> MDRFQIGDEQLLRFYQLKTINPTHSWAQDSSKLNNEEATSNELGVETSFDILKDFKYGNQISIDKESRAYLNDESLSYIRDPLNGQEMSKELQHLPNDSMRLNYLVNSKQFNVKAFLRDMHKQDSFNDLNNSLDRLDSDIQDQSIHLKQLVGKNFTKYVKIKNKLDQIYKEFDEKTNEKNQCDSPKENQINVESLNKKVDEVIRTTTFKLKPLMDNYQKILNYQATKKFIELNKFYFNLPKSLKRCLTNNDFNEFIIEYSKGLTLRRRFNQSSDASQSLVIKRIWTQIENLLVTYKDLIWNSLINSNFNIDQPQETILSLFSKLLNLENFINNNQRESESGNKNTTSSSNENPILRWMSIKMNGFQNELNELSGHMISKIIHSQRLILQNNTNQDKSQGCVELSYYLKINQLFQIISDTGKDSEGLKSTVEPNKVNTISGTSYLNLNCQPSSQGLTDSPTIIEMWLLILKYIN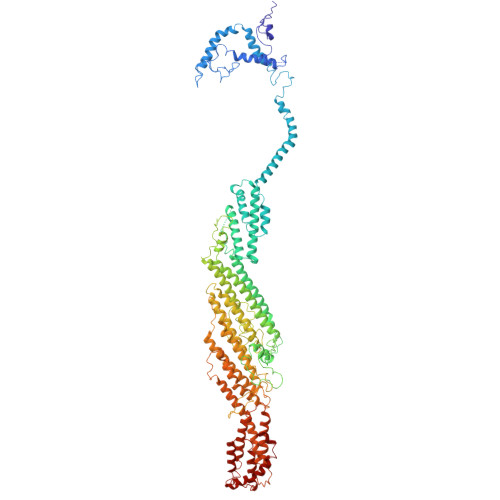DLWKICDQFIEFWEHIEKFLDGTYQNSIINEKRKENILIGDSNIIESYQKSLILKEEQINEVRLKGEEFITSVSQNLISFFTSSQSSLPSSLKDSTGDITRSNKDSGSPLDYGFIPPNCNGLSCLRYLPKIVEPILKFSTELAQLNITTNGITICRNTLSTIINRCVGAISSTKLRDISNFYQLENWQVYETVTFSSKSQDSSKNLTFEYGVTQFPEIVTSFQEVSIKTTRDLLFAYEKLPIINGISVVSYPSKQLLTGIEIQQIISMEAVLEAILKNAAKDKDNPRNSHTILTLTNLQYFRECAFPNILQYFDDAFEWNLASKNLELFSLLSKMESSIFGNYLSDLKINLRDTLEEKFHEINWPMYTSNSFRVGDYIIEALMILIVVHSECFRIGPQLIHKILIETQIFIARYLFEAFKPYVGNLSNDGSLQIIVDLEFFQKVMGPLLEKDTEATLRACLQNCFQNDTNRLQKCINEINPIVSANLKRTAIQFAAFS>MGHHHHHHHHHHSSGHENLYFQGQQDKLVLRVDGILNELDAQVLEGILTRLNGVRQFRLDRISGELEVVFDPEV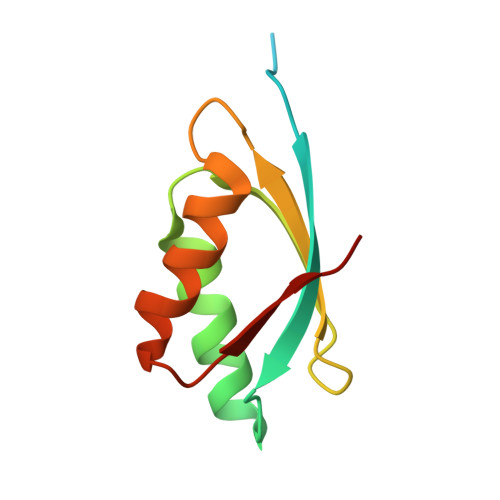VSSRSLVDGIEEDGFGKFKLRVMSPY[2x]> MLFDLRPKTRREDIFDREEESRKLEESLENYPLTLLLGIRRVGKSSLLRAFLNERPGILIDCRELYAERGHITR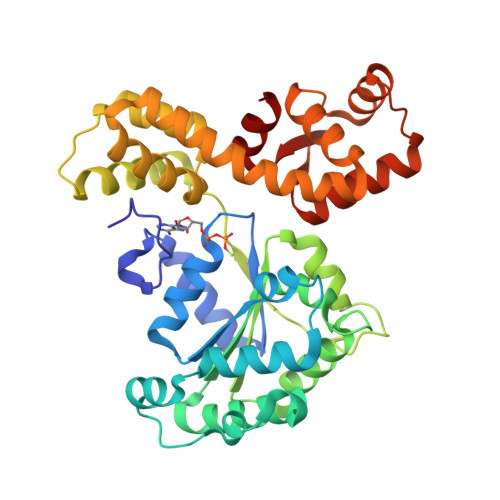EELIKELQSTISPFQKFQSKFKISLNLKFLTLEPRKLSLREVFRELNDLGEELGEFIVAFDEAQYLRFYGSRGGKELLALFAYAYDSLPNLKIILTGSEVGLLHDFLKITDYESPLYGRIAGEVLVKPFDKDTSVEFLKRGFREVNLDVPENEIEEAVELLDGIPGWLVVFGVEYLRNGDFGRAMKRTLEVAKGLIMGELEELRRRSPRYVDILRAIALGYNRWSLIRDYLAVKGTKIPEPRLYALLENLKKMNWIVEEDNTYKIADPVVATVLRI2-[3-[(1~{R})-1-[(2~{S})-1-[(2~{S})-2-(5-chloranylthiophen-2-yl)-2-(3,4,5-trimethoxyphenyl)ethanoyl]piperidin-2-yl]carbonyloxy-3-(3,4-dimethoxyphenyl)propyl]phenoxy]ethanoic 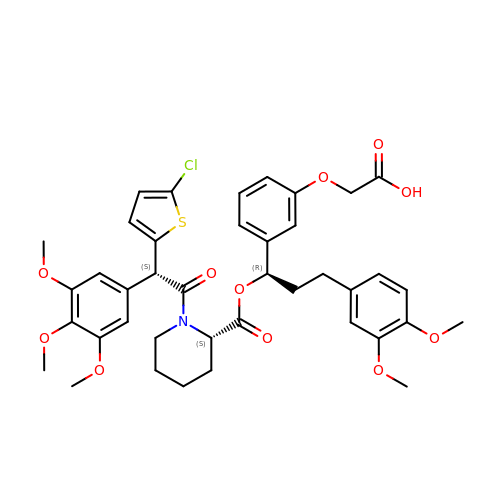acid | C40 H44 Cl N O11 S | DJMQVDNYVWNBAD-DBWZWNDFSA-N>EQARPADDALAALGAQLFVDPALSRNATQSCATCHDPARAFTDPREGKAGLAVSVGDDGQSHGDRNTPTLGYAALVPAFHRDANGKYKGGQFWDGRADDLKQQAGQVMLNPVEMAMPDRAAVAARLRDDPAYRTGFEALFGKGVLDDPERAFDAAAEALAAYQATGEFSPFDSKYDRVMRGEEKFTPLEEFGYTVFITWNCRLCHMQRKQGVAERETFTNFEYHNIGLPVNETAREASGLGADHVDHGLLARPGIEDPAQSGRFKVPSLRNVAVTGPYMHNGVFTDLRTAILFYNKYTSRRPEAKINPETGAPWGEPEVARNLSLAELQSGLMLDDGRVDALVAFLETLTDRRYEPLLEESRAAQKDHHHHHH[2x];>ADAPAGTDPRAKWVPQDNDIQACDYWRHCSIDGNICDCSGGSLTNCPPGTKLATASWVASCYNPTDGQSYLIAYRDCCGYNVSGRCPCLNTEGELPVYRPEFANDIIWCFGAEDDAMTYHCTISPIVGKASHHHHHH[2x];>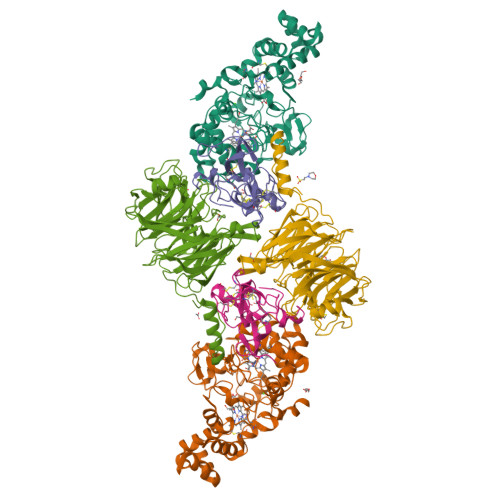[2x]QDAPEAETQAQETQGQAAARAAAADLAAGQDDEPRILEAPAPDARRVYVNDPAHFAAVTQQFVIDGEAGRVIGMIDGGFLPNPVVADDGSFIAHASTVFSRIARGERTDYVEVFDPVTLLPTADIELPDAPRFLVGTYPWMTSLTPDGKTLLFYQFSPAPAVGVVDLEGKAFKRMLDVPDCYHIFPTAPDTFFMHCRDGSLAKVAFGTEGTPEITHTEVFHPEDEFLINHPAYSQKAGRLVWPTYTGKIHQIDLSSGDAKFLPAVEALTEAERADGWRPGGWQQVAYHRALDRIYLLVDQRDEWRHKTASRFVVVLDAKTGERLAKFEMGHEIDSINVSQDEKPLLYALSTGDKTLYIHDAESGEELRSVNQLGHGPQVITTADMG> MGHHHHHHHSMDITFTADKFARRAEEAAPVAVKPPRNPEFGIFLNNRYLLHNGEGLPKPKDVKETYPECKWRKYGQWAWLDENNVQCYLGPSYKYHAYSPAKNFDPVPSI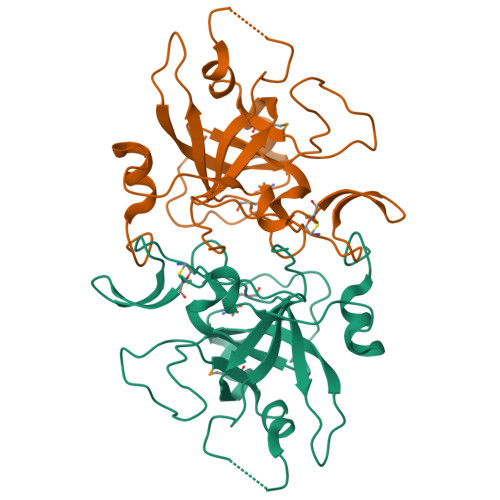QRGACADTANPQDFPQGIPRYTISVPYLYFNNFYDRRCKVRALVKVPQTDKEKEHWIQAWVVEHNGGNWSTKSGDLGPNGPQEGIMLDTKLYPKFLNSGDKDIGVLPNKVEWFFLDINTIG>[4x]MKKVIIAGNGPSLKEIDYSRLPNDFDVFRCNQFYFEDKYYLGKKCKAVFYNPSLFFEQYYTLKHLIQNQEYETELIMCSNYNQAHLENENFVKTFYDYFPDAHLGYDFFKQLKDFNAYFKFHEIYFNQRITSGVYMCAVAIALGYKEIYLSGIDFYQNGSSYAFDTK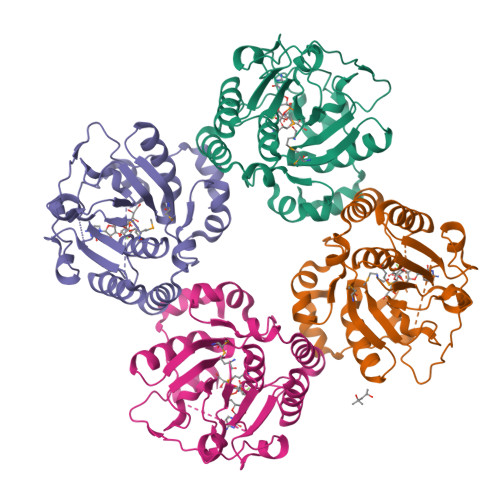QKNLLKLAPNFKNDNSHYIGHSKNTDIKALEFLEKTYKIKLYCLCPNSLLANFIELAPNLNSNFIIQEKNNYTKDILIPSSEAYGKFSKNIN> MKDFEFFAPKTLEEAKGLLHQYKDVPPAIIAGGTDLVIEINDRWEKPDVVIDIKKLKELEYIRVEENTIHIGALSTFTQIENHPFIRSHVRALYKAASQVGSPQIRNLGTIGGNLSTSSVAGDG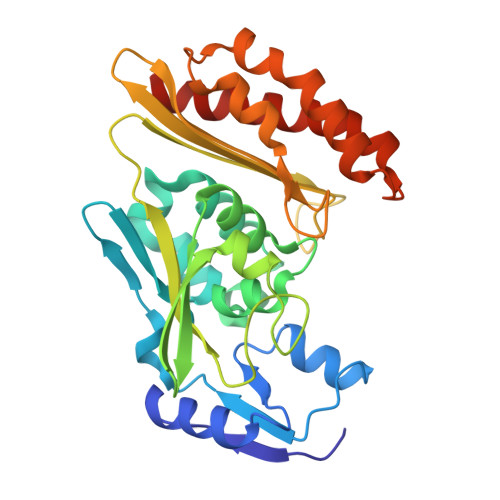VSAMTTLDATVVLESVRGTRQMKLTDFFDGEGFKRRNALEADEIMTEVIIDRPDAHSASAFYKLAKRKSLAISVIGGGMAVKVDDAGVCTWASMRGGCIGRYPLHFKQAEEMLVGAPLTMETMEATLPILHDTVYDMARARPSVLYKKESVQGVFKKLFVDILDQLEGGCNE> EDMPVERILEAELAVEPKTETYVEANMGLNPSSPNDPVTNICQAADKQLFTLVEWAKRIPHFSELPLDDQVILLRAGWNELLIASFSHRSIAVKDGILLATGLHVHRNSAHSAGVGAIFDRVLTELVSKMRDMQMDKTELGCLRAIVLFNPDSKGLSNPAEVEALREKVYASLEAYCKHKYPEQPGRFAKLLLRLPALRSIGLKCLEHLFFFKLIGDTPIDTFLMEMLEA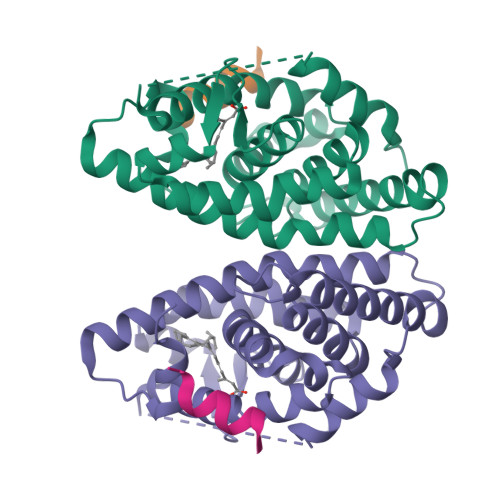PHQMT;> KHKILHRLLQDSS> AEAGITGTWYNQLGSTFIVTAGADGALTGTYESAVGNAESRYVLTGRYDSA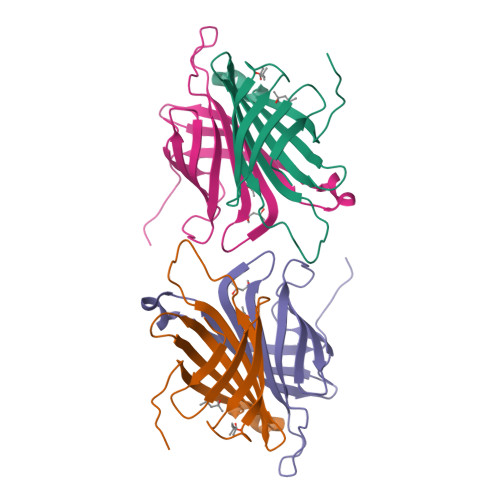PGRGDSPGSGTALGWTVAWKNNYRNAHSATTWSGQYVGGAEARINTQWLLTSGTTEANAWKSTLVGHDTFTKVKPSAAS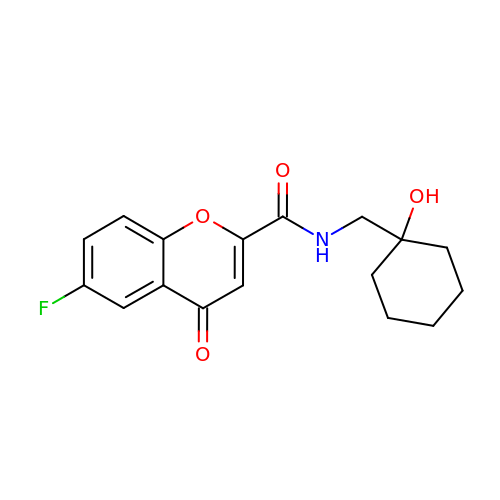6-fluoranyl-~{N}-[(1-oxidanylcyclohexyl)methyl]-4-oxidanylidene-chromene-2-carboxamide | C17 H18 F N O4 | PHMBHONIMDVOKO-UHFFFAOYSA-N> SLGLLTALIRKGPSEEWKFKISEVASDLEVPWSIAPLGGGRYLVTERPGRLVLISPSGKKLVASFDVANVGEAGLLGLALHPEFPKKSWVYLYASYFAEGGHIRNRV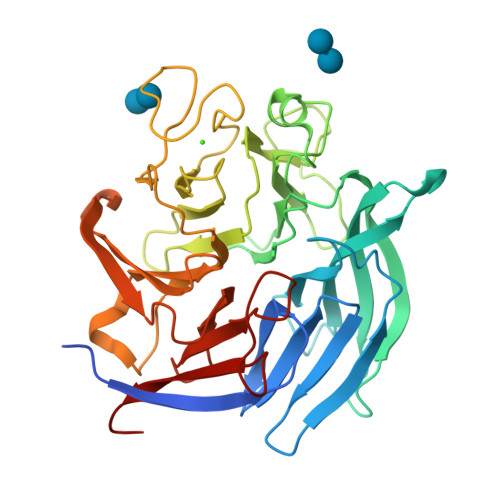IRGRLDGSTFKLKEVKTLIDGIPGAYIHNGGRIRFGPDGMLYITTGDAADPRLAQDLSSLAGKILRVDEEGRPPADNPFPNSPIWSYGHRNPQGIDWHRASGVMVATEHGPVGHDEVNIILKGGNYGWPLATGKAGRGEFVDPVIDTGSETWAPSGASFVHGDMFPGLRGWLLIACLRGSMLAAVNFGDNMEVRKISTFFKNVFGRLRDVVIDDDGGILISTSNRDGRGSLRAGDDKILKIVSEQHT trans-N-{(1S)-1-[4-(3-amino-2H-indazol-6-yl)pyridin-2-yl]-2-phenylethyl}-4-(aminomethyl)cyclohexanecarboxamide | C28 H32 N6 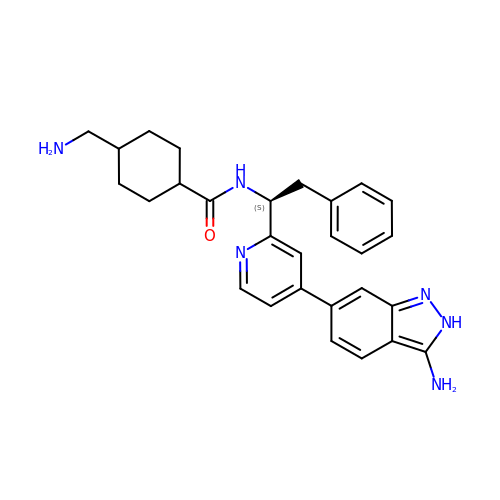O | ABPMTNUZKFZRKL-DYLHXGEVSA-N>GSHMSNITYVKGNILKPKSYARILIHSCNCNGSWGGGIAYQLALRYPKAEKDYVEVCEKYGSNLLGKCILLPSYENSDLLICCLFTSSFGGSSHGEKQSILNYTKLALDKLKTFREAKDKTRTSEDSIGDYLNGHIKYPIGEYKLEMPQINSGIAGV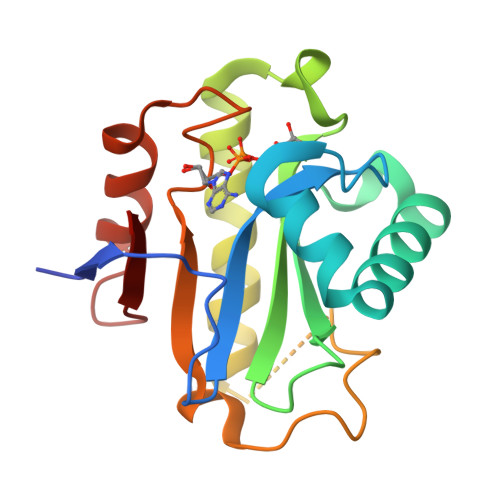PWKETERVLEEFSGDMSFTVYQL[2x]> LLLLLLLLLLLLL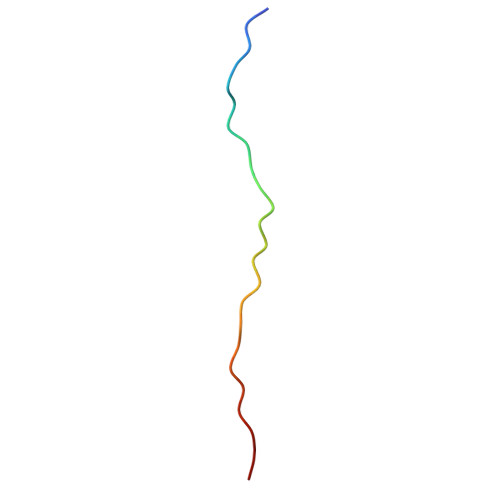LLLLLLLLLLL>[4x]MASWSHPQFEKGANQPQSWEARAETYSLYGFTDMPSVHQRGTVVVTHGEGPYIVDVHGRRYLDANSGLWNMVAGFDHKGLIEAAKAQYDRFPGYHAFFGRMSDQTVMLSEKLVEVSPFDNGRVFYTNSGSEANDTMVKMLWFLHAAEGKPQKRKILTRWNAYHGVTAVSASMTGKPYNSVFGLPLPGFIHLTCPHYWRYGEEGETEAQ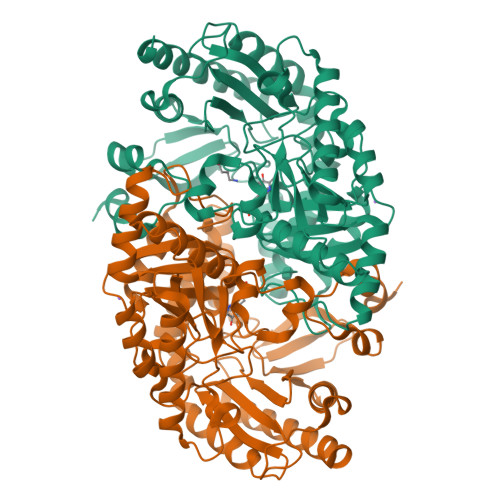FVARLARELEDTITREGADTIAGFFAEPVMGAGGVIPPAKGYFQAILPILRKYDIPMISDEVICGFGRTGNTWGCLTYDFMPDAIISSKNLTAGFFPMGAVILGPDLAKRVEAAVEAIEEFPHGFTASGHPVGCAIALKAIDVVMNEGLAENVRRLAPRFEAGLKRIADRPNIGEYRGIGFMWALEAVKDKPTKTPFDANLSVSERIANTCTDLGLICRPLGQSIVLCPPFILTEAQMDEMFEKLEKALDKVFAEVA(N6,N6)-methyl,benzyl-C2-chloro-(alpha,beta)-methylene-ADP | C19 H24 Cl N5 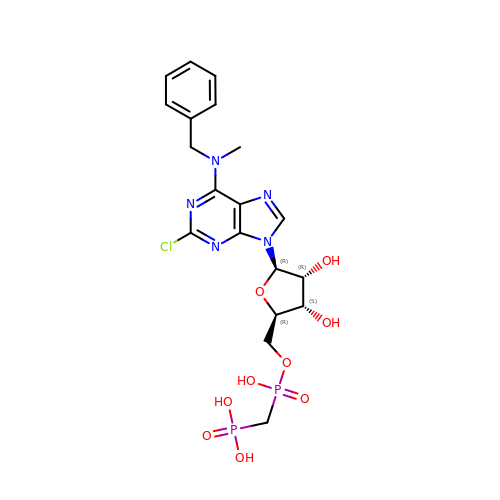O9 P2 | NRCRRUYZIFHEBT-SCFUHWHPSA-N The phosphate acyltransferase PlsX is one of the few proteins known to localize to RIFs in B. subtilis, which are present in a punctate pattern and stained with a high specificity with the lipid analog indocarbocyanine dye DiIC12. This enzyme catalyzes the first chemical step in phospholipid biosynthesis by converting acyl–acyl carrier protein (ACP) and phosphate into acyl phosphate and is essential in a large subset of bacteria. PlsX is an obvious peripheral membrane protein because it was over-expressed and purified as a cytosol protein10 and yet was consistently observed to associate with the membrane.

B. subtilis PlsX was crystallized in the presence of the product analog palmitoyl phosphoramide and the crystal structure was determined at 2.30 Å resolution. However, the product analog was not found in the solved structure, in which the asymmetric unit contains two largely symmetric subunits in a mushroom architecture with a four-helix bundle stem formed at the dimeric interface. The structure is closely similar to the previously solved structure of the same protein with a root-mean-squared deviation of 0.56 Å over all comparable Cα carbon atoms, forming two symmetric large cavities suspected to be the active sites at the dimeric interface (circled in Fig. 1a). The only obvious difference with the previous structure lies in a 13-residue fragment (residues 250–262) at the exposed end of the helix bundle stem. The 13-residue fragment is structurally different in the two subunits of the dimeric structure. It is comprised of a 9-residue (residues 253–261) α-helix and a 2-residue loop in chain B and a largely random coil loop in chain A. Interestingly, the 9-residue α-helical peptide in chain B is amphipathic with Thr253, Thr255, and Lys257 at the interface and Leu254, Leu258, and Ala261 forming the nonpolar surface together with the hydrophobic part of the interfacial residues. The N-terminus of the α-peptide is connected to the end of one vertical helix through the 2-residue loop (Thr251 and Ser252) and its C-terminus is connected to another vertical helix of the four-helix bundle stem via a one-residue sharp turn (Val262). This amphipathic α-peptide was formed in the crystal likely due to the presence of the product analog, palmitoyl phosphoramide, which is an anionic detergent by nature. By mutating the interfacial residues of the amphipathic peptide and determining their effects on the subcellular localization, we showed that this α-peptide is indeed responsible for the RIFs localization through direct interaction with the membrane.

>[2x]MRIAVDAMGGDHAPKAVIDGVIKGIEAFDDLHITLVGDKTTIESHLTTTSDRITVLHADEVIEPTDEPVRAVRRKKNSSMVLMAQEVAENRADACISAGNTGALMTAGLFIVGRIKGIDRPALAPTLPTVSGDGFLLLDVGANVDAKPEHLVQYAIMGSVYSQQVRGVTSPRVGLLNVGTEDKKGNELTKQTFQILKETANINFIGNVEARDLLDDVADVVVTDGFTGNVTLKTLEGSALSIFKMMRDVMTSTLTSKLAAAVLKPKLKEMKMKMEYSNYGGASLFGLKAPVIKAHGSSDSNAVFHAIRQAREMVSQNVAALIQEEVLEHHHHHH4-[2-[2-(4-methoxyphenyl)ethylamino]ethyl]benzene-1,2-diol | C17 H21 N O3 | 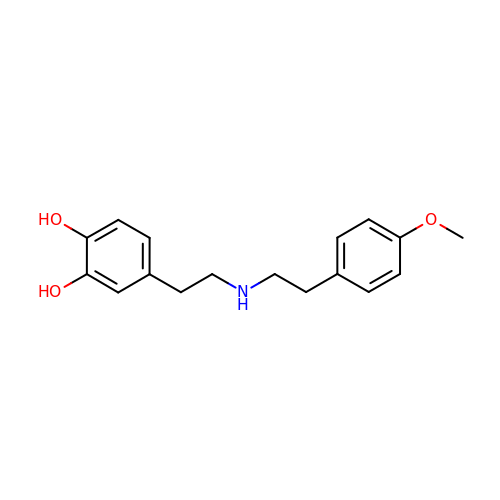YUWZXUMQIZRXEN-UHFFFAOYSA-N> MNVPFWTEEHVRATLPERDAESHKGTYGTALLLAGSDDMPGAALLAGLGAM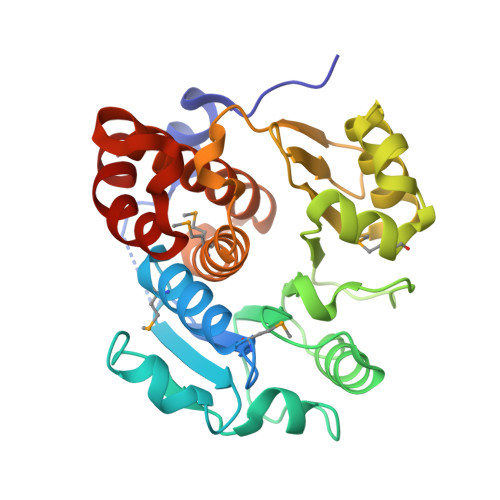RSGLGKLVIGTSENVIPLIVPVLPEATYWRDGWKKAADAQLEETYRAIAIGPGLPQTESVQQAVDHVLTADCPVILDAGALAKRTYPKREGPVILTPHPGEFFRMTGVPVNELQKKRAEYAKEWAAQLQTVIVLKGNQTVIAFPDGDCWLNPTGNGALAKGGTGDTLTGMILGMLCCHEDPKHAVLNAVYLHGACAELWTDEHSAHTLLAHELSDILPRVWKRFE> MGHHHHHHMELKASEFGVVLSVDALKLS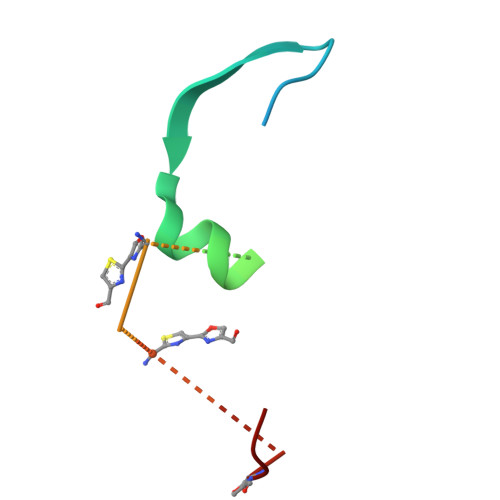RQSPLGVGIGGGGGGGGGGSCGGQGGGCGGCSNGCSGGNGGSGGSGSHI>MFIVNTNVPRASVPDGFLSELTQQLAQATGKPPQYIAVHVVPDQLMAFGGSSEPCALCSLHSIGKIGGAQNRSYSKLLCGLL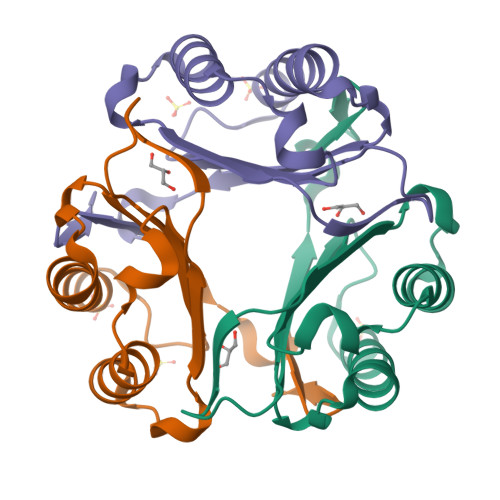AERLRISPDRVYINYYDMNAANVGWNNSTFA[3x]3-(4-methoxy-3-methylphenyl)propanoic 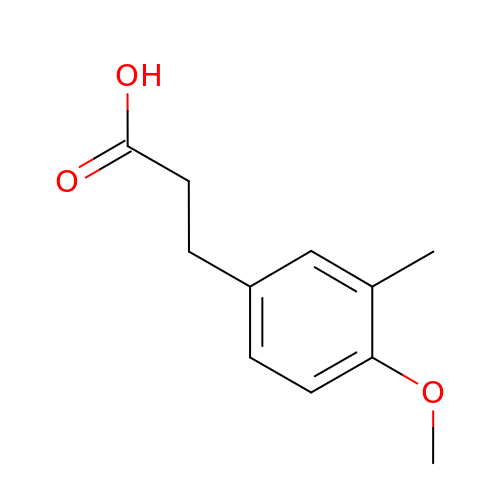acid | C11 H14 O3 | ZATPJYSLVGVGGY-UHFFFAOYSA-N> DQDKIEALSSKVQQLERSIGLKDLAMADLEQKVLEMEASTYDGVFIWKISDFARKRQEAVAGRIPAIFSPA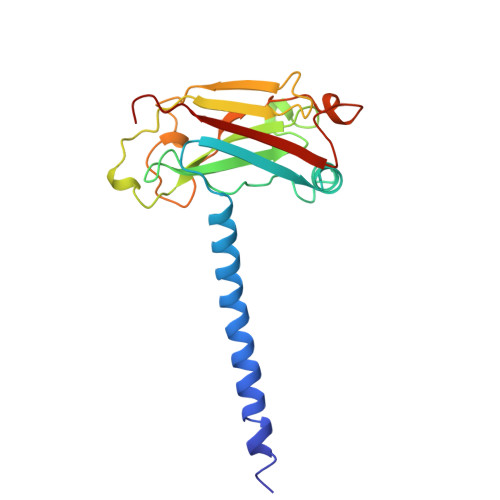FYTSRYGYKMCLRIYLNGDGTGRGTHLSLFFVVMKGPNDALLRWPFNQKVTLMLLDQNNREHVIDAFRPDVTSSSFQRPVNDMNIASGCPLFCPVSKMEAKNSYVRDDAIFIKAIVDLTGL>MTAQRSTTNPVLEPLVAVHREIYPKADLSILQRAYEVADQRHASQLRQSGDPYITHPLAVANILAELGMDTTTLVAALLHDTVEDTGYTLEALTEEFGEEVGHLVDGVTKLDRVVLGSAAEGETIRKMITAMARDPRVLVIKVADRLHNMRTMRFLPPEKQARKARETLEVIAPLAHRLGMASVKWELEDLSFAILHPKKYEEIVRLVAGRAPSRDTYLAKVRAEIVNTLTASKIKATVEGRPKHYWSIYQKMIVKGRDFDDIHDLVGVRILCDEIRDCYAAVGVVHSLWQPMAGRFKDYIAQPRYGVYQSLHTTVVGPEGKPLEVQIRTRDMHRTAEYGIAAHWRYKEAKGRNGVLHPHAAAEIDDMAWMRQLLDWQREAADPGEF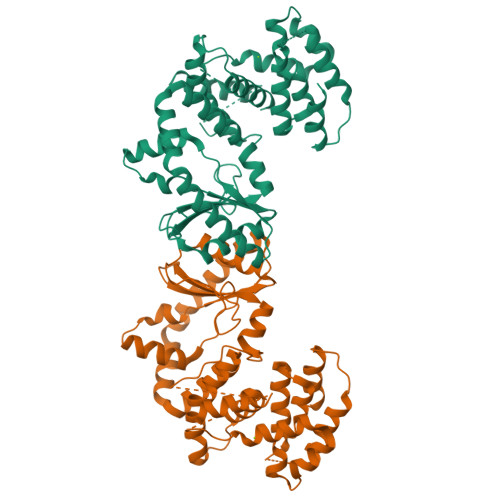LESLRYD[4x]> MKYFTVFTALTALFAQASASAIPAVRSTLTPRQNTTASCANSATSRSCWGEYSIDTNWYDVTPTGVTREYWLSVENSTITPDGYTRSAMTFNGTVPGPAIIADWGDNLIIHVTNNLEHNGTSIHWHGIRQLGSLEYDGVPGVTQCPIAPGDTLTYKFQVTQYGTTWYHSHFSLQYGDGLFGPLIINGPATADYDEDVGVIFLQDWAHESVFEIWDTARLGAPPALENTLMNGTNTFDCSASTDPNCVGG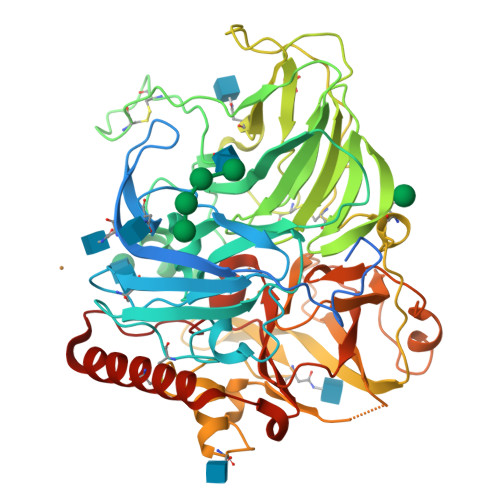GKKFELTFVEGTKYRLRLINVGIDSHFEFAIDNHTLTVIANDLVPIVPYTTDTLLIGIGQRYDVIVEANAAADNYWIRGNWGTTCSTNNEAANATGILRYDSSSIANPTSVGTTPRGTCEDEPVASLVPHLALDVGGYSLVDEQVSSAFTNYFTWTINSSSLLLDWSSPTTLKIFNNETIFPTEYNVVALEQTNANEEWVVYVIEDLTGFGIWHPIHLHGHDFFIVAQETDVFNSDESPAKFNLVNPPRRDVAALPGNGYLAIAFKLDNPGSWLLHCHIAWHASEGLAMQFVESQSSIAVKMTDTAIFEDTCANWNAYTPTQLFAEDDSGI> MSKFDTSALEAFVRHIPQNYKGPGGVVAVVKDGEVVLQHAWGFADLRTRTPMTLDTRMPICSVSKQFTCAVLLDAVGEPELLDDALEAYLDKFEDERPAVRDLCNNQSGLRDYWALSVLCGADPEGVFLPAQAQSLLRRLKTTHFEPGSHYSYCNGNFRILADLIEAHTGRTLVDILSERIFAPAGMKRAELISDTALFDECTGYEGDTVRGFLPATNRIQWMGDAGICASLNDMIAWEQFIDATRDDESGLYRRLSGPQTFKDGVAAPYGFGLNLHETGGKRLTGHGGALRGWRCQRWHCADERLSTIAMFNFEGGASEVAFKLMNIALGVSSSEVSRVEADSAWFGSWLDDETGLVLSLEDAGHGRMKARFGTSPEMMDVVSANEARSAVTTIRRDGETIELVRASENLRLSMKRVKGEAKHDIIGRYHSDELDADLLLVSEGGAIYGAFEGFLGKSDMYPLYSVGSDV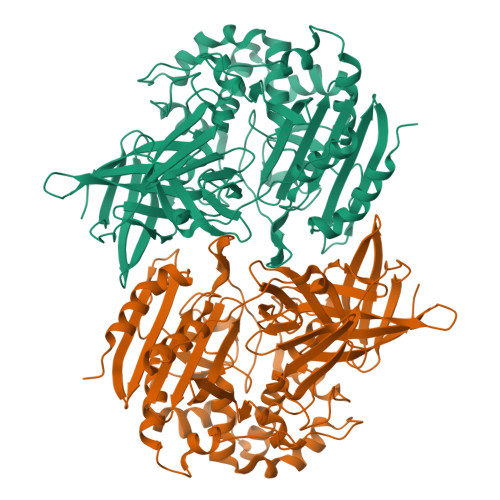WLLPVQRSMDAPSPGEWKLVFRRDDKGEITGLSVGCWLARGVEYRRVQP> MTPPKAEKRPYPITTHGDTRVDDYYWLRDDERTDPQVLDYLQAENAFTDAALKPQQALRETLYEEMVARIPQQEHSVPYVRHGYRYQTRFEPGNEYAIYVRQPQAESEHWDTLIDGNQRAEQREFYTLGGLEVSPDNQKLAVAEDFLSRRQYDIRFKNLSDDSWTDEVLENTSGSFEWANDSATVYYVRKHAKTLLPYQVYRHVVGTDPQLDELIYEEQDDTFYVGLEKTTSDRFILIHLSSTTTSEILLLDADRADSTPQMFVPRRKDHEYGIDHYHQHFYIRSNKDGKNFGLYQSEQADEAQWQTLIAPRIEVMLEGFSLFRDWLVVEERSEGLTQLRQIHWQSGEVKRIAFDDPTYTTWLAYNPEPETELLRYGYSSMTTPTTLYELNLDSDERVMLKQQEVKNFTPENYRSERVWVKARDGVEVPVSLVYRHDSFARGTNPLMVYGYGSYGSSMDPAFSASRLSLLDRGFVFVLAHIRGGGELGQLWYEDGKLFKKQNTFNDFIDVTEALIAQGYGDAKRVFAMGGSAGGLLMGAVINQAPELFNGIVAQVPFVDVVTTMLDESIPLTTGEYDEWGNPNQQAYYDYILQYSPYDQVKAQDYPHMLVTTGLHDSQVQYWEPAKWVAKLRELKTDDRQLLLYTDMDSGHGGKSGRFKAYEDIALEYAFILALAE

Oligopeptidases B (OpBs, EC 3.4.21.83) are trypsin-like serine peptidases that belong to the prolyl oligopeptidase (POP) family (S9 family) of clan SC. Endopeptidases from the S9A subfamily cleave peptide bonds on the carbonyl side of either proline (POPs) or basic amino acid residues (OpBs). The catalytic domain includes the α/β-hydrolase fold, which is canonical for serine proteases and is located at the C-terminal part of the molecule, and the N-terminal loop, which is divided from the α/β hydrolase fold by the regulatory β-propeller domain. The β-propeller domain consists of seven blade-shaped beta sheets arranged around the central axis according to the open Velcro topology (no connection between first and last blades) and restricts access of substrates larger than 3 kDa to the catalytic triad located in the interdomain cavity.

The structure of wild type SpOpB bound to tosyl-L-lysine chloromethyl ketone (TCK) was determined at 2.2 Å resolution. The unit cell dimensions of the SpOpB-TCK crystal were 75.529 Å × 89.660 Å × 108.650 Å, a crystallographic space group was P2(1)2(1)2(1), an asymmetric unit contained a monomer in a crystal lattice. A clear electron density for one molecule of covalently bound TCK, which is a modified lysine residue tosylated at the N-terminus and chloromethylated at the C-terminus, was observed from the 2mFo-DFc difference map in the active site. The closed state of SpOpB was associated with covalent binding of a single TCK molecule to the catalytic S532 and H652 residues. The binding to the OG atom of S532 occurs through the hemiacetal carbon atom of TCK, and to the NE2 atom of H652, it occurs through the methylene group of TCK. Despite the presence of spermine in the crystallization mixture, no spermine molecules were found in the crystal structure. According to these criteria, the newly obtained structure of SpOpB-TCK indeed represents the closed state of the enzyme. The SpOpB-TCK complex can be considered as an analogue of the transition state in the proteolytic reaction catalyzed by S532. The position of the lysine side chain of TCK coincides with the position of the P1 arginyl of AIP and the position of the tosyl ring coincides with that of the P2 valine of AIP. Both the lysine amino group of TCK and the arginyl guanidino group of AIP interact with E576 and E607 carboxyl groups of SpOpB and TbOpB, respectively. The carbonyl group of P2 valine of AIP is H-bound to the R650-NH1 atom of TbOpB, while the similarly located O1S atom of TCK is H-bound to the Q619-NE2 of SpOpB.> IVGGYTCGANTVPYQVSLNSGYHFCGGSLINSQWVVSAAHCYKSGIQVRLGEDNINVVEGNEQFISASKSIVHPSYNSETYNNDIMLIKLKSAASLNSRVASISLPTSCASAGTQCLISGWGNTKSSGTSYPDVLKCLKAPILSD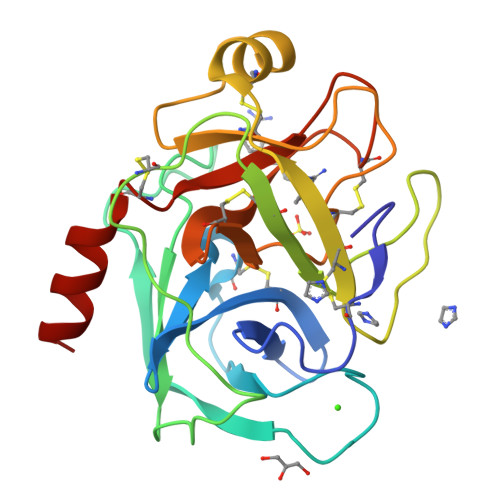SSCKSAYPGQITSNMFCAGYLEGGKDSCQGDSGGPVVCSGKLQGIVSWGSGCAQKNKPGVYTKVCNYVSWIKQTIASN>ETGMPQYSTFHSENRDWTFNHLTVHRRTGAVYVGAINRVYKLTGNLTIQVAHKTGPEEDNKACYPPLIVQPCSEVLTLTNNVNKLLIIDYSENRLLACGSLYQGVCKLLRLDDLFILVEPSHKKEHYLSSVNKTGTMYGVIVRSEGEDGKLFIGTAVDGKQDYFPTLSSRKLPRDPESSAMLDYELHSDFVSSLIKIPSDTLALVSHFDIFYIYGFASGGFVYFLTVQPETPDGMAINSAGDLFYTSRIVRLCKDDPKFHSYVSLPFGCTRAGVEYRLLQAAYLAKPGEALAQAFNISSDEDVLFAIFSKGQKQYHHPPDDSALCAFPIRAINLQIKERLQSCYHGEGNLELNWLLGKDVQCTKAPVPIDDNFCGLDINQPLGGSTPVEGLTLYTTSRDRLTSVASYVYNGYSVVFVGTKSGKLKKIRADGPPHGGVQYEMVSVFKDGSPILRDMAFSINQLYLYVMSERQVTRVPVESCEQYTTCGECLSSGDPHCGWCALHNMCSRRDKCQRAWEANRFAASISQCMSLEVHPNSISVSDHSRLLSLVVNDAPNLSEGIACAFGNLTEVEGQVSGSQVICISPGPKDVPVIPLDQDWFGLELQLRSKETGKIFVSTEFKFYNCSAHQLCLSCVNSAFRCHWCKYRNLCTHDPTTCSFQEGRINVSEDCPQLVPTEEILIPVGEVKPITLKARNLPQPQSGQRGYECVLSIQGAVHRVPALRFNSSSVQCQNSSYQYDGMDISNLAVDFAVVWNGNFIIDNPQDLKVHLYKCAAQRESCGLCLKADHKFECGWCSGERRCTLHQHCPSTSSPWLDWSSHNVKCSNPQITEILTVSGPPEGGTRVTIHGVNLGLDFSEIAHHVQVAGVPCTPIPGEYIIAEQIVCEMGHAVIGTTSGPVRLCIGECKPEFMTKSHQQYTFVNPSVLSLSPIRGPESGGTMVTITGHYLGAGSSVAVYLGNQTCEFYGRSMNEIVCVSPPSSNGLGPVPVSVSVDRARVDSSLQFEYIDDPRVQRIEPEWSITSGHTPLTITGFNLDVIQEPRVRVKFNGKESVNVCTVVNTTTLTCLAPSLTSDYRPGLDTVERPDEFGFLFNNVQSLLIYNDTKFIYYPNPTFELLSPTGILDQKPGSPIILKGKNLCPPASGGAKLNYTVMIGETPCTVTVSETQLLCEPPNLTGQHKVMVHVGGMVFSPGSVSVISDGGSRTKHHHHHH[4x]

Class A plexins (PlxnAs) act as semaphorin receptors and control diverse aspects of nervous system development and plasticity, ranging from axon guidance and neuron migration to synaptic organization. Plexins are large type 1 transmembrane proteins comprising typically ten domains in their extracellular segment, a single membrane spanning region that is predicted to be helical and a conserved, cytoplasmic region that contains a GTPase-activating protein (GAP) domain with a Rho GTPase-binding domain insert. All our PlxnA ectodomain structures show autoinhibitory, intermolecular “head-to-stalk” (domain 1 to domain 4-5) interactions, which are confirmed by biophysical assays, live cell fluorescence microscopy, and cell-based and neuronal growth cone collapse assays. This work reveals a 2-fold role of the PlxnA ectodomains: imposing a pre-signaling autoinhibitory separation for the cytoplasmic domains via intermolecular head-to-stalk interactions and supporting dimerization-based PlxnA activation upon ligand binding.

We determined crystal structures of the full extracellular segments of mouse PlxnA1, PlxnA2, and PlxnA4 from eight crystal forms providing a total of 13 independent structures that range in maximum resolution from 4 to 10 Å. In five out of 13 full extracellular structures all ten domains are resolved whereas in the other eight structures some of the C-terminal domains were not modeled due to fragmentary or absent electron density. This indicates that some flexibility is present in the extracellular segment of plexins. Some flexibility in the stalk is evident on comparison of the 13 different structures and contributes to the ring diameter ranging from 84 Å to 99 Å. All our PlxnA full ectodomain crystal structures have an intermolecular plexin–plexin interface in common. This interface is formed by blades 1–3 of the sema domain of one plexin molecule and the outer side of domains 4-5 (PSI2-IPT2) from the ring of a second plexin. The residues in this interface are conserved among vertebrate PlxnAs but much less among all plexins, suggesting that this plexin–plexin interaction may be an important functional feature of PlxnAs.> MQSMILFAAALMGAAVNGFVLPRTDDPDCETKATDCGSTSNIKYTVVKGDTLTSIAKKFKSGICNIVSVNKLANPNLIELGATLIIPENCSNPDNKSCVSTPAEPTETCVPGLPGSYTIVSGDTLTNISQDFNITLDSLIAANTQIENPDAIDVGQIITVPVCPSSQCEAVGTYNIVAGDLFVDLAATYHTTIGQIKALNNNVNPSKLKVGQQIILPQDCKNVTTAVA

The leaf mold fungus Cladosporium fulvum abundantly secretes the LysM-containing effector protein Ecp6 (for extracellular protein 6; Bolton et al., 2008) during colonization of its host tomato. Ecp6 acts as a scavenger of chitin fragments and thus prevents recognition of the fungus by host immune receptors. The three LysMs of Ecp6 (LysM1–LysM3) share the typical βααβ-fold, with LysM1 being separated by a long and flexible linker from a compact and rigid body formed by LysM2 and LysM3. The composite LysM1–LysM3 binding site shows ultra-high chitin-binding affinity, thus explaining how LysM effectors outcompete plant host receptors for chitin binding.

Here, we report the crystal structure of Ecp6 to a resolution of 1.6 Å, revealing a novel mechanism for chitin binding by LysMs that developed in fungi, involving substrate-induced intrachain dimerization of two LysM domains to form a buried intramolecular chitin-binding groove. The structure was determined by single-wavelength anomalous dispersion (SAD) and refined to a resolution of 1.6 Å with an Rwork and Rfree of 20.3% and 22.5%, respectively. The structure model comprises nearly the complete mature protein sequence, from amino acid residues 7 to 195. Ecp6 has a tightly packed structure that is stabilized by four disulfide bridges, and two spatially close glycosylation sites (Asn104 and Asn193) were identified. Unexpectedly, the calculated 2Fo−Fc map showed a well-defined electron density for a bound chitin tetramer (GlcNAc)4 in a large interdomain groove between LysM1 and LysM3 (∼16 Å long and ∼11 Å across its widest points), although the protein crystallized in the absence of exogenously added chitin. The chitin oligomer was likely co-purified with Ecp6 and derived from the cell wall of the P. pastoris expression system. Evidently, LysM1 and LysM3 of Ecp6 cooperate to bring two chitin-binding regions together, composing a novel type of binding groove in which one chitin tetramer is nearly completely buried and engaged in many noncovalent interactions, including 12 hydrogen bonds. Specifically, the groove is shaped by the amino acids 20GDTLT24 and 46PNLIEL51 of LysM1 and 150GDLFV154 and 176PSKL179 of LysM3. The chitin binding is further strengthened by noncovalent interactions among proximate residues on the complementary surfaces of LysM1 (N45 and 47NLIE50) and LysM3 (150GDLFVD155). Furthermore, the solute-exposed ends of the chitin tetramer in the structure suggest that longer oligomers can also be bound to the groove, in which case four GlcNAc units of a chitin oligomer make direct contact with the protein while the remaining parts of the molecule protrude into the solvent.>MLKNGMRPIHPGEILREEFQKEMGFSAAALARALGVATPTVNNILRERGGVSADMALRLSICLDTTPEFWLNLQTAFDLRTAEQQHGDEIIGSVQRLVA[2x];>MHHHHHHIRSFSCADTEALFTTGKTRRGSDIKSVAERKLAMLDAATELRDLRSPPGNRLESLSGNRADQHSI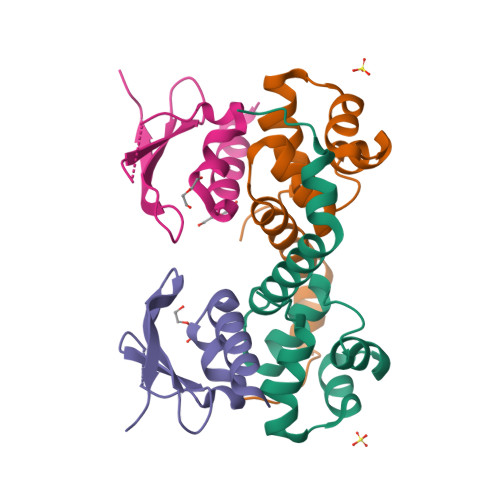RVNDQWRLCFTWTEHGPVNVEIVDYH[2x]> GSMGY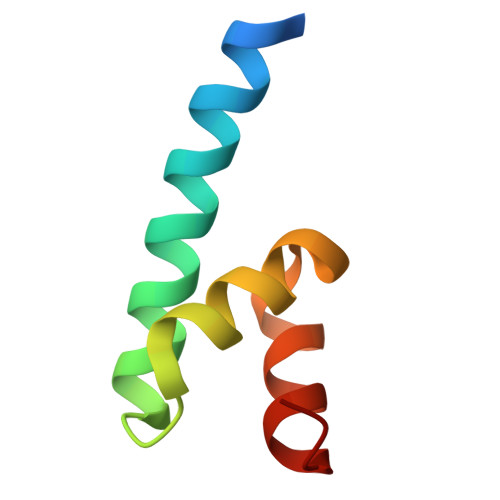RGSENLYFQGQLNAMAHQIQEMFPQVPYHLVLQDLQLTRSVEITTDNILEGRI>[2x]MVNTEEDGLPRLIDAIEEASKIPAKRRQTPIKPTIEKLTTHLYTHGASPDSLLRLADLLTLRNHLDQASL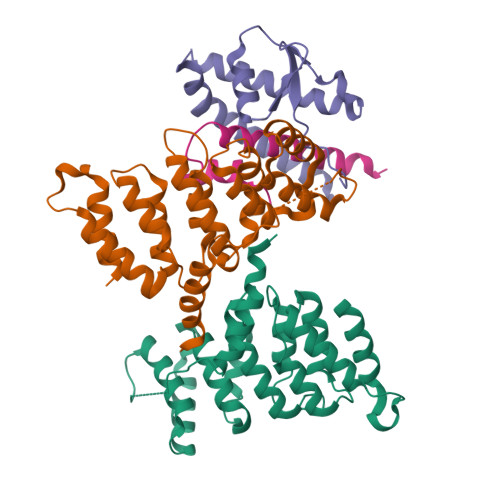AAITRNLYPSSTVSDEVVLRFIGALGHGQLKPTLALQALFLRWLVMVYHLLENPGVLGQVYGVLFDLLDTAAIRPQLCHLLALVTRRKHVRPFRIQAILTLSRQTGGDPNLTGLLRVFKNYYPEIIVGDATKGRASAFKHPDPQWRQHLDEIQQRRSEA;> RQKDEWAKKTSSLMKQLDWFIGEHLGAMLAAEELGGPVVGELMEIDPDDLSAGFNAHGKLKKATSQPDLDRRQRRIDDIWGPQDEQGQAHKRKRGADEALAASAEMRDLIEQLMNKLVEAGGDNSATYVEIPRESAAARFLVRSKVAMFHPNDARRLRLVDFGRDLDD;> HEAEMKSNRRRWRIMKGAASAIVAGSGIDWVRDERLRDLVLDLPD Here, we describe the identification, biochemical and structural characterization of a new D-amino acid transaminase from Haliscomenobacter hydrossis (Halhy). The new enzyme is strictly specific towards D-amino acids and their keto analogs; it demonstrates one of the highest rates of transamination between D-glutamate and pyruvate. TAs catalyze the stereoselective transfer of an amino group from an amino acid/amine to a keto acid/ketone/aldehyde, producing a new chiral amino acid/amine and a new keto compound. Transaminases are usually homodimers, comprising two symmetrical active sites formed by the residues of both subunits.

Furthermore, Halhy is attractive as a potential biocatalyst because of its stability at 40–50 °C. We succeeded in obtaining the crystal structure of the holo form of Halhy with a resolution of 2.0 Å. The Halhy subunit consists of two α/β domains: a small domain (residues 1–114) and a large domain (residues 128–281), connected by an interdomain loop (residues 115–127). The contact analysis showed that Halhy is a homodimer in the crystal. The residues from both subunits form two symmetrical active sites in the dimer, with the PLP molecule covalently bound via a Schiff base to the catalytic K143. Additionally, PLP is coordinated by the conserved among TAs of PLP fold type IV residues: E176, forming a hydrogen bond with N1 atom of pyridine ring and R52, I202, T203, and T239, forming hydrogen bonds with the phosphate moiety of PLP. The phenyl oxygen atom of PLP forms a hydrogen bond with Y147 located on the α-helix of the large domain. Similar to the known TAs of PLP fold type IV, the active site of Halhy can be divided into two pockets: the O-pocket (near the phenyl moiety of PLP) and the P-pocket (near the phosphate moiety of PLP). The O-pocket of Halhy is confined by the side chains of residues F33, R28*, R90, and R179, forming a positively charged patch. Instead, in Halhy, the side chains of R28* and R90 are directed into the “carboxylate trap” place and could bind the α-carboxylic group of substrates. There are no positively charged residues in the P-pocket of Halhy, and the γ-carboxylic group can be coordinated by the side chain of S238 and the backbone nitrogen atoms of the β-turn 238STIK241.

> MGSDKIHHHHHHENLYFQGHMIKYYNINGQQVPVENATLHVSDLSILRGYGIFDYFLAREGHPLFLDDYLNRFYRSAAELYLEIPFDKAELRRQIYALLQANEVREAGIRLVLTGGYSPDGYTPVNPNLLIMMYDLPASAWEFSAQGIKIITHPFQRELPEVKTINYSTGIRMLKTIKERGATDLIYVDQGEWIRESARSNFFLVMPDNTIVTADEKILWGITRRQVIDAAREAGYAVEERRIHITELDQAREAFFTSTIKGVMAIGQIDDRVFGDGTIGKVTQELQDLFVGKVKAYLETC>[2x]MNTIAWLGRLVIERIRGIGVAALMLLQIIFSLPSAGGFGRFVYQMHRVGVMSLLIITVSGLFIGLVLGLQGYSILVNVGSESMLGTMVSLTLLRELAPVVAALLFAGRAGSALTAEIGSMKQSEQLASMEMIGVDPLKQIVSPRLWAGIVSLPMLTVIFAAIGIVGGKLVGVDFLGVDEGSFWSGMQNNVQFGHDVVNGIIKSIVFALLCTWIAVFQGYACDPTPEGIATAMTRTVVYSSLCVLGFDFVLTAVMFGGI;>MMNNKTPLSTQSLIEVKNLSFNRG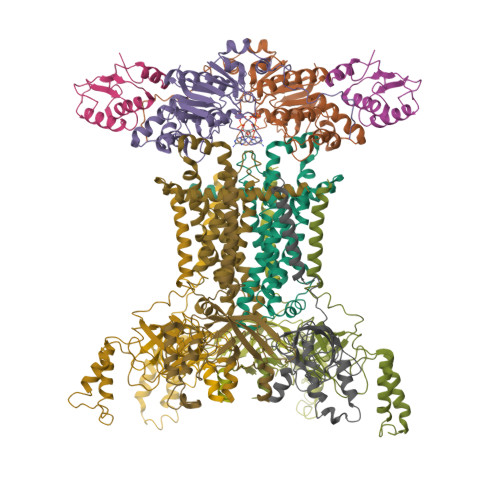ERVIYDNISLNIRRGQITAIMGPSGTGKTTLLRLIGGQLVPDQGEVLLDGKDIAQMSRQELFAARARMGMLFQSGALFTDMSVYENVAFPIRAHTKLSENLIAELVALKLESVGLRGTEQLMPTELSGGMNRRVALARAIALDPDLIMYDEPFAGQDPIVKGVLTRLIRSLREALDLTTIIVSHDVPETLSIADYIYVVAEGKIQGEGTPEELQAYASPFVKQFLTGSAEGPVEYQFSHQAYLDNEVRP[2x];>VVQYLNQELVVSGKIDFENAEQQYQAGLAIIKKQTSFPLIVDLKQLEHGNTLALAVLVQWLRQTPQKSGLHFKNVPEKMLKIIQACHLQEDLHLVLEHHHHHH[2x];>[6x]MKSRTSELAVGIFVIIFGIALFFLAMKVSGLVGTNLSDGYTMKAQFDNVNGLKPRAKVTMSGVTIGRVDSITLDPVTRLATVTFDLDGKLTSFNAEQLKEVQKNALDELRYSSDYTQATPAQQKTMEQQLISNMNSITSIDEDAYIMVATNGLLGEKYLKIVPGGGLNYLKRGDTISNTQGTMDLEDLISKFITGGGAGKVAAGSSSAEEKAPASTDSSAQP> MKKAVINGEQIRSISDLHQTLKKELALPEYYGENLDALWDALTGWVEYPL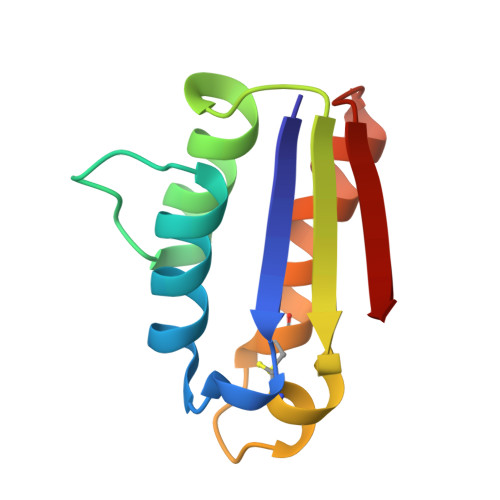VLEWRQFEQCKQLTENGCESVLQVFREAKAEGADITIILS1-(2-hydroxyethyl)-1H-pyrazole-4-carboxamide 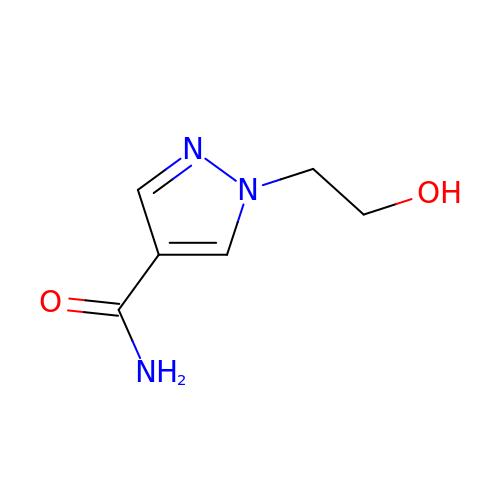| C6 H9 N3 O2 | LHYHSUSQLBMWFV-UHFFFAOYSA-N> FTANIKGLTQASRNANDGISIAQTTEGALNEINNNLQRVRELAVQSANSTNSQSDLDSIQAEITQRLNEIDRVSGQTQFNGVKVLAQDNTLTIQVGANDGETIDIDLKQINSQTLGLDTLNVQQKYKVSDTAATVTGYADTTIALDNSTFKASATGLGGTDQKIDGDLKFDDTTGKYYAKVTVTGGTGKDGYYEVSVDKTNGEVTLAGGATS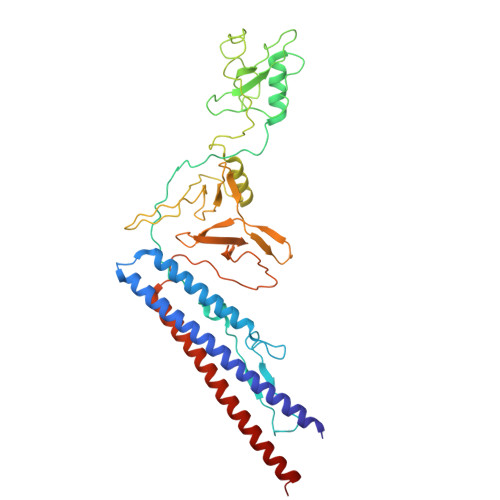PLTGGLPATATEDVKNVQVANADLTEAKAALTAAGVTGTASVVKMSYTDNNGKTIDGGLAVKVGDDYYSATQNKDGSISINTTKYTADDGTSKTALNKLGGADGKTEVVSIGGKTYAASKAEGHNFKAQPDLAEAAATTTENPLQKIDAALAQVDTLRSDLGAVQNRFNSAITNLGNTVNNLTSARSRI> HHHHHHMAKKVNWYVSCSPRSPEKIQPELKVLANFEGSYWKGVKGYKAQEAFAKELAALPQFLGTTYKKEAAFSTRDRVAPMKTYGFVFVDEEGYLRITEAGKMLANNRRPKDVFLKQLVKWQYPSFQHKGKEYPEEEWSINPLVFVLSLLKKVGGLSKLDIAMFCLTATNNNQVDEIAEEIMQFRNEREKIKGQNKKLEFTENYFFKRFEKIYGNVGKIREGKSDSSHKSKIETKMRNARDVADATTRYFRYTGLFVARGNQLVLNPEKSDLIDEIISSSKVVKNYTRVEEFHEYYGNPSLPQFSFETKEQLLDLAHRIRDENTRLAEQLVEHFPNVKVEIQVLEDIYNSLNKKVDVETLKDVIYHAKELQLELKKKKLQADFNDPRQLEEVIDLLEVYHEKKNVIEEKIKARFIANKNTVFEWLTWNGFIILGNALEYKNNFVIDEELQPVTHAAGNQPDMEIIYEDFIVLGEVTTSKGATQFKMESEPVTRHYLNKKKELEK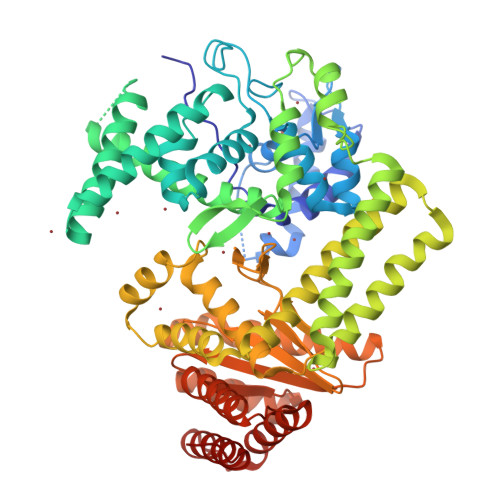QGVEKELYCLFIAPEINKNTFEEFMKYNIVQNTRIIPLSLKQFNMLLMVQKKLIEKGRRLSSYDIKNLMVSLYRTTIECERKYTQIKAGLEETLNNWVVDKEVRF>[3x]AQVINTFDGVADYLQTYHKLPDNYITASEAQALGWVASKGNLADVAPGKSIGGDIFSNREGK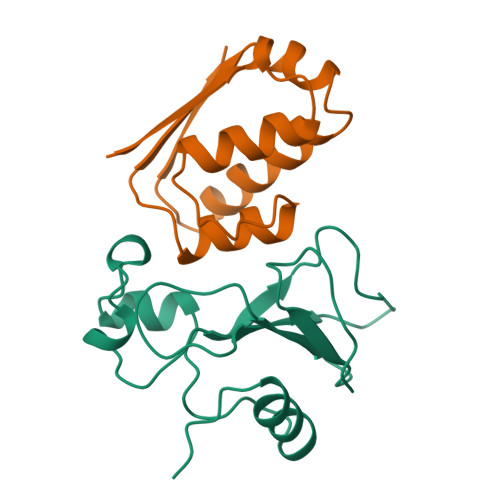LPGKSGRTWREADINYTSGFRNSDRILYSSDWLIYKTTDHYQTFTKIR;>[3x]MKKAVINGEQIRSISDLHQTLKKELALPEYYGENLDALWDCLAGWVEYPLVLEWRQFEQSKQLTENGAESVLQVFREAKAEGCDITIILS>GSSHHHHHHLEVLFQGPVNALVSHLLVVEPEKLYAMPDPAGPDGHLPAVATLSDLFDREIVVTISWAKSIPGFSSLSLSDQMSVLQSVWMEVLVLGVAQRSLPLQDELAFAEDLVLDEEGARAAGLGELGAALLQLVRRLQALRLEREEYVLLKALALANSDSVHIEDAEAVEQLREALHEALLEY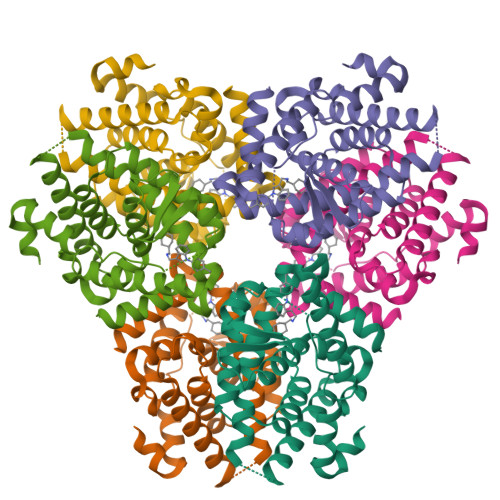EAGRAGPGGGAERRRAGRLLLTLPLLRQTAGKVLAHFYGVKLEGKVPMHKLFLEMLEAMMD[2x]> MEQKQQSERLGTEAIPKLLRSLSIPAMIGMFVMALYNVVDTIFISYAVGIEGVAGVTIAFPIMMIMMSMAGALGIGGASVISRRLGERRGEEANQVFGNILTVILVLSVIGFISAFTLLGPALQLFGATSVTQGYATDYLFPILLGSIFFFFAFAANNIIRSEGNATFAMVTMIVPAVLNILLDVLFIFGLNMGVLGASIATVIAQASVTGLVLRYFLTGKSTLSLHWSDLRMKGSVIKEVCLVGLPAFVQQSSASLMMIAINSMLLRFGSDFYVGVFGLVQRIMMFVMMPMMGIMQAMQPIVGYNYGAKQYSRLRETVMLGFKVATIFSIGIFALLMLFPEALLRVFTADREVIQAGVSAMHILFCVTFLIGAQIVAGGLYQSLGKPKQALILSLS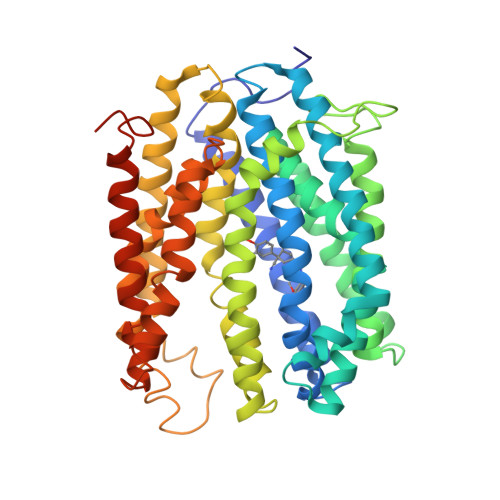RQIIFLIPLVLILPHIFGLSGVWWAFPIADVLSFILTVVLLYRDRNVFFLKTKEERELDLVKTASST> VDPRAKWQPQDNDIQACDYWRHCSIDGNICDCSGGSLTNCPPGTKLATASWVASCYNPT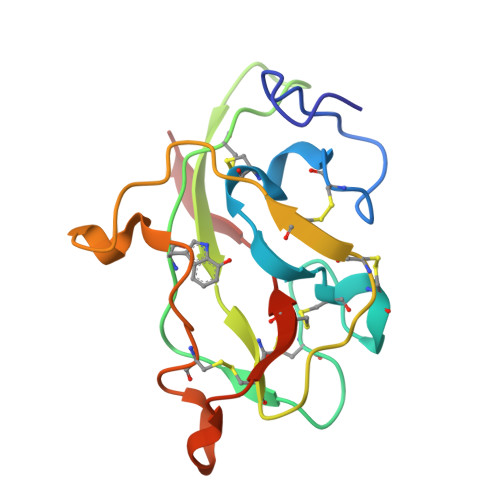DGQSYLIAYRDCCGYNVSGRCPCLNTEGELPVYRPEFANDIIWCFGAEDDAMTYHCTISPIVGKA>MNTRVAIIGAGPCGLAQLRAFQSAAAKGAAIPELVCFEKQSDWGGMWNYTWRTGVDEHGEPVHGSMYRYLWSNGPKECLEFADYTFDEHFGRPIGSYPPREVLWDYIKGRVEKAGVRDYIRFNTAVRQVSYDETSGLFSVTVQDHSNNRVYTETFDYVVNACGHFSTPNTPYFEGFERFGGRVLHAHDFRDALEFKDKDILVVGSSYSAEDIGSQCYKYGARSITSCYRSAPMGYQWPQNWEEKPLLQRVDSDTAWFADGSHKRIDAIILCTGYQHHFPFLPDSLRLITENRLWPLKLYKGIFWEDNPKFLYLGMQDQWYSFNMFDAQAWYARDVILGRISLPGKAEMQAENQAWREREEKLQTAQEMFEFQGSYIQHLIDATDYPSFDIQAVNETFLAWKH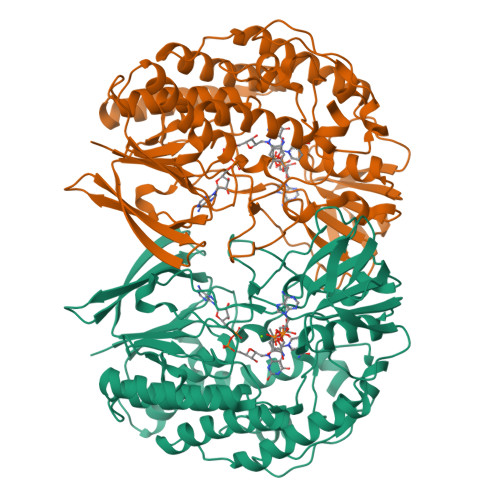DKYEDIMGYRNKCYRSLMTGTLATPHHTPWLDALDDSLEAYLQETPRLKSAV[2x]>[2x]SMKQYEHVTRDLNPEDFWEIIGELGDGAFGKVYKAQNKETSVLAAAKVIDTKSEEELEDYMVEIDILASCDHPNIVKLLDAFYYENNLWILIEFCAGGAVDAVMLELERPLTESQIQVVCKQTLDALNYLHDNKIIHRDLKAGNILFTLDGDIKLADFGVSAKNTRTIQRRDSFIGTPYWMAPEVVMCETSKDRPYDYKADVWSLGITLIEMAEIEPPHHELNPMRVLLKIAKSEPP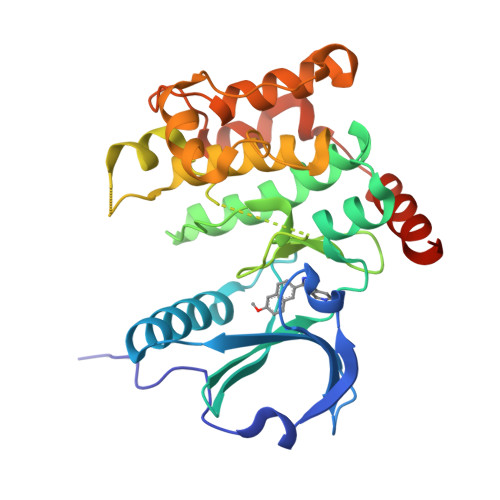TLAQPSRWSSNFKDFLKKCLEKNVDARWTTSQLLQHPFVTVDSNKPIRELIAEAKAEVTEEVEDGKE>GGACUCGACU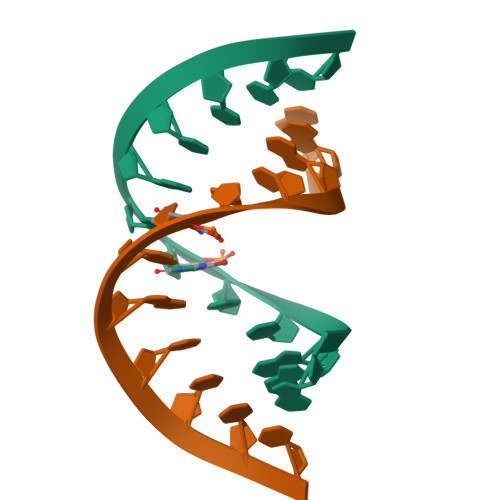CC[2x]>GPDIKVTPGTSELVEQILALLSRYLSSYIHVLNKFISHLRRVATLRFERTTLIKFVKKLRFYNDSVLSYNASEFINEGKNELDPEADSFDKVILPIASMFVKSVETFDLLNYYLTQSLQKEILSKTLNEDLTLTAESILAIDDTYNHFVKFSQWMIESLRIGSNLLD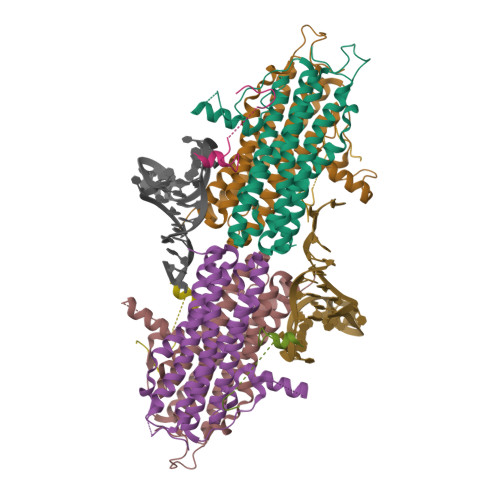LEVVQFAIKSADEDGTNIGETDNIFLQEILPVNSEEEFQTLSAAWHSILDGKLSALDEEFDVVATKWHDKFGKLKNGGSGGGGSGGSSNGNSSNNKRRSFYTASPLLSSGSIPKSASPVLPGVKRTASVRKPSSSSSKTNVTHNNDPSTSPTISVPPGVTR[8x]> AMAKETAAAKFERQHMDSSTSAASSSNYCNQMMKSRNLTKDRCKPVNTFVHESLADVQAVCSQKNVA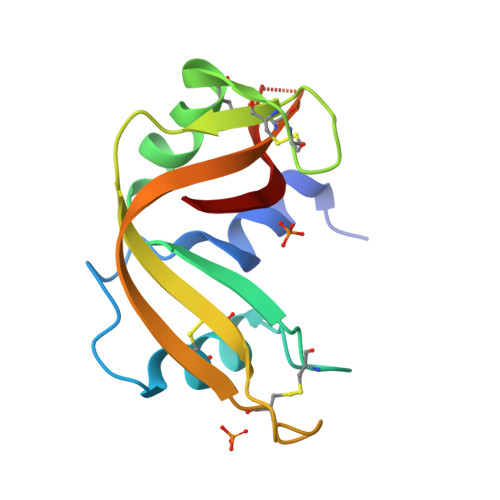CKNGQTNCYQSYSTMSITDCRETGSSKYPNCAYKTTQANKHIIVACEGGQQQQQQQQQQGNPYVPVAFDASV3-(5-AMINO-3-IMINO-3H-PYRAZOL-4-YLAZO)-BENZOIC 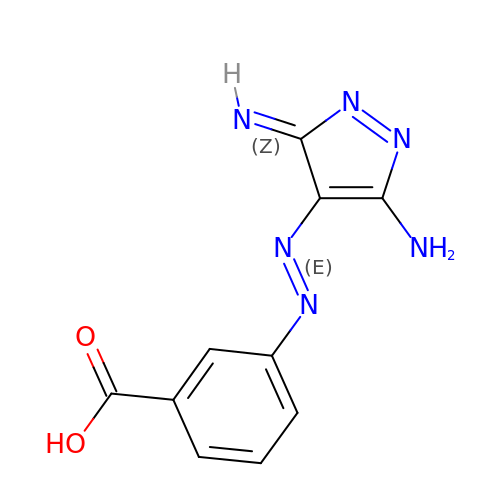ACID | C10 H8 N6 O2 | PIUSHRUXZPMNPD-KBABRGLLSA-N> MATPSMMPQWAYMHIAGQDASEYLSPGLVQFARATDTYFSLGNKFRNPTVAPTHDVTTDRSQRLTLRFVPVDREATTYLYKARFTLAVGDNRVLDMASTYFDIRGVLDRGPSFKPYSGTAYNSLAPKGAPNPSQWETKEKQGTTGGVQQEKDVTKTFGVAATGGINITNQGLLLGTDETAENGKKDIYADKTFQPEPQVGEENWQENEAFYGGRALKKDTKMKPCYGSFARPTNEKGGQAKF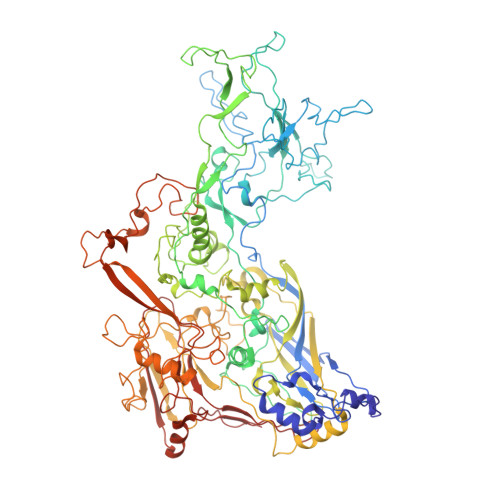KPVNEGEQPKDLDIDFAYFDVPGGSPPAGGSGEEYKADIILYTENVNLETPDTHVVYKPGTSDNSSEINLVQQSMPNRPNYIGFRDNFVGLMYYNSTGNMGVLAGQASQLNAVVDLQDRNTELSYQLLLDSLGDRTRYFSMWNSAVDSYDPDVRIIENHGVEDELPNYCFPLNGTGTNSTYQGVKITNGNDGAEESEWEKDDAISRQNQICKGNVYAMEINLQANLWKSFLYSNVALYLPDSYKYTPANVKLPANTNTYEYMNGRVVAPSLVDAYINIGARWSLDPMDNVNPFNHPRNAGLRYRSMLLGNGRYVPFHIQVPQKFFAIKNLLLLPGSYTYEWNFRKDVNMILQSSLGNDLRVDGASVRFDSVNLYATFFPMAHNTASTLEAMLRNDTHDQSFNDYLSAANMLYPIPAKATNVPISIPSRNWAAFRGWSFTRLKTKETPSLGSGFDPYFVYSGSIPYLDGTFYLNHTFKKVSIMFDSSVSWPGNDRLLTPNEFEIKRSVDGEGYNVAQCNMTKDWFLVQMLSHYNIGYQGFHVPEGYKDRMYSFFRNFQPMSRQVVDEINYKDYKAVTLPFQHNNSGFTGYLAPTMRQGQPYPANFPYPLIGQTAVPSVTQKKFLCDRVMWRIPFSSNFMSMGALTDLGQNMLYANSAHALDMTFEVDPMDEPTLLYLLFEVFDVVRVHQPHRGVIEAVYLRTPFSAGNATT> FNCTSSSATVHWLGDKPTYHAGVTFGLPWPQGKYRPQETSFSLTGDTEDKSELQSWATGYWADGSLKWTAHAIAESNQIYDQYTVTASSLGCVKSSSSSSESSAPNSSIVVTDNSDALTVNTGEVAVSFPKGGNVIIGDIKTKSGKVIGANGRLVLQSQDSVPDNFDNRANSPIQYSNFDGNINEVFVNQTSARTLVTVRGNHTVTDGTDHDPWLPFVVRFYLYANSATIKVMHSIVFDGDENDFITGLGIRFDVPLKGEEYYDRHIRFAGVDGGIFNEAVQGITGLRRDPGEEIRAAQFAGQKLADTETWEPRVSTRLKWIPTWADYGLTQLTADGFGLKKRTKAGQSWVNIPSGTRAEGLAYLGGATQGGLAVGLRDFWKRYPVGLDISNAASDTGELTLWLYSPAAEPLDLRPFHDGLGQDGYEDQLDALEITYEDWEPGFDTPYGIARTSEVYLFAFDQTPTSDKLASLTAYMNDPPVLVAEPKYIHETQALGEYWA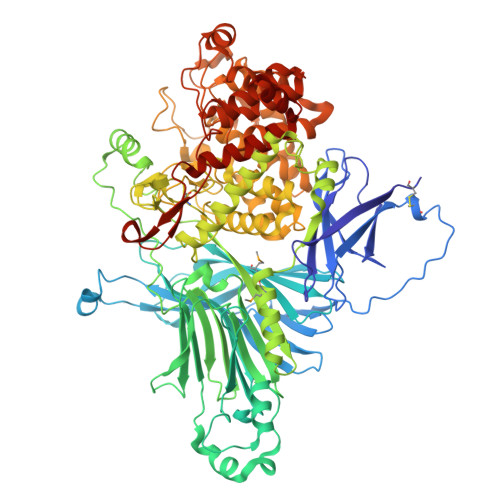LPGSASPAAATLEDRLQFIFDFYKGQIEQRRWYGFLDYGDFMHTYDPDRHTWRYDVGGYAWDNSELSPDLFFWLYFLRTGSKDAYRFAEALTRHTGEVDVYHIGDWKGLGTRHGVQHWSDSAKQARISQPQYRKYFFYLSGGDERVGELLEELLDTDKTYGELDPQRKVRTDGWEPSPNSTVSFGLGTDWSGLAAGWLIEWERRGPRWEEAKTKLTNTIAGIANLTNGFVTGSGLYDPVTWTLGPPPSDPGNRGNVSISHLNAVFGLPEVVSEAIAYLADDIPKGFKQAWLDYCYYYHASASEQKDRYGVSFSKISLLQAHSRLAAYAAYETKNKTLALRAWKDFYASDGLLPDAPWNITHVDGSDVLVPVDEAAWLATNDIAQYGLAVIQNLAYVSDSLDDYQSLE> MKIGIVGLGRVGSSTAFALLMKGFAREMVLIDVDKKRAEGDALDLIHGTPFTRRANIYAGDYADLKGSDVVIVAAGVPQKPGETRLQLLGRNARVMKEIARNVSKYAPDSIVIVVTNPVDVLTYFFLKESGMDPRKVFGSGTVLDTARLRTLIAQHCGFSPRSVHVYVIGEHGDSEVPVWSGAMIGGIP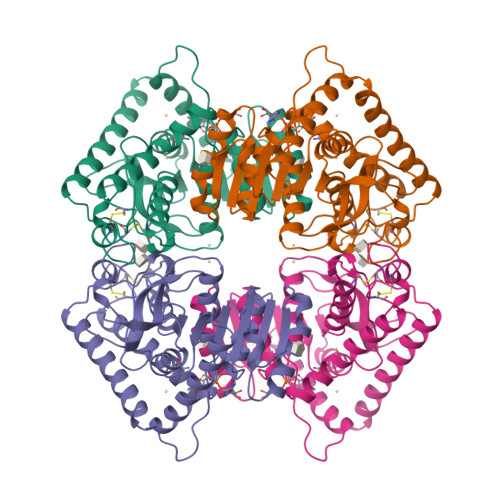LQNMCQVCQKCDSKILENFAEKTKRAAYEIIERKGATHYAIALAVADIVESIFFDEKRVLTLSVYLEDYLGVKDLCISVPVTLGKHGVERILELNLNEEELEAFRKSASILKNAINEITAEENKHQNTSG>ATQGVFTLPANTRFGVTAFANSSATQTVKVLVNNETAATFTGQSTNNAVIGSQVLNSGGGGKVQIQVSVNGRSSD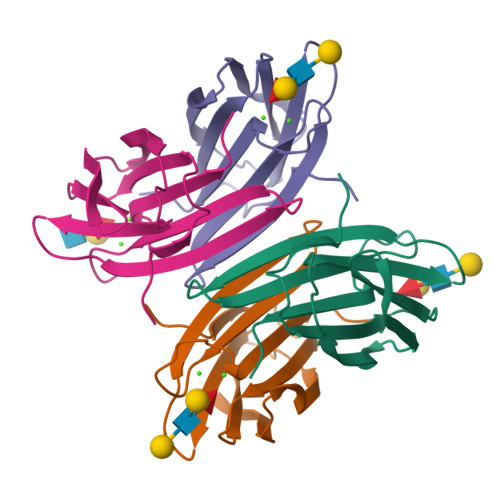LVSAQVILANELNVALVGSEDSTDNDYNDAVVVINWPLG[4x]>[4x]MNNNDIEYNAPSEIKYIDVVNTYDLEEEA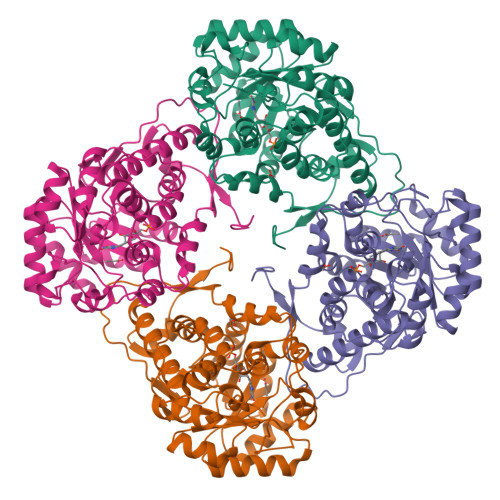SKVVPHGGFNYIAGASGDEWTKRANDRAWKHKLLYPRLAQDVEAPDTSTEILGHKIKAPFIMAPIGAHGLAHATKEAGTARAVSEFGTIMSISAYSGATFEEISEGLNGGPRWFQIYMAKDDQQNRDILDEAKGDGATAIILTADSTVSGNRDRDVKNKFVYPFGMPIVQRYLRGTAEGMSLNNIYGASKQKISPRDIEEIAAHSGLPVFVKGIQHPEDADMAIKAGASGIWVSNHGARQLYEAPGSFDTLPAIAERVNKRVPIVFDSGVRRGEHVAKALASGADVVALGRPVLFGLALGGWQGAYSVLDYFQKDLTRVMQLTGSQNVEDLKGLDLFDNPYGYEY>[3x]MVRLLLTSFQHPSMAQFIGGKRVAYIPDAARSYADAP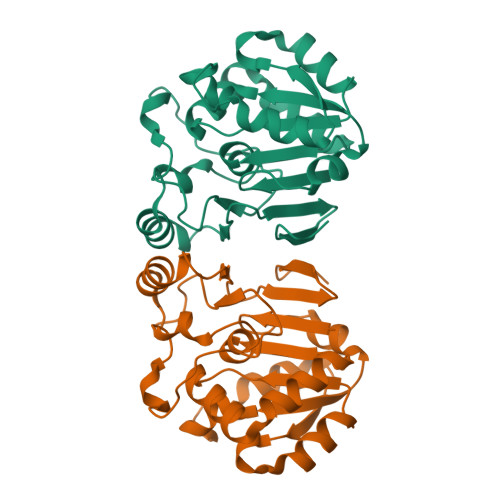FVQKEREGLEKQGLELINLPLSHTDLAAVETTLNAVDGVYVAGGETFDLLQVLRSTGSDKVITRRVRQGLPYIGCSAGSVVAGPTIEAVSLMDSPDIAPDLKDYTGLGLTELAVIPHASGSISQFPIETIADTVRTYGERWPLCLLRDGQALWIEDGEVRLLNLEHHHHHH>[6x]DRHHHHHHGSVTQRTFKLDYSRDRFLKDGQPFRYISGSIHYFRIPRFYWEDRLLKMKMAGLNAIQMYVPWNFHEPQPGQYEFSGDRDVEHFIQLAHELGLLVILRPGPYICAEWDMGGLPAWLLEKQSIVL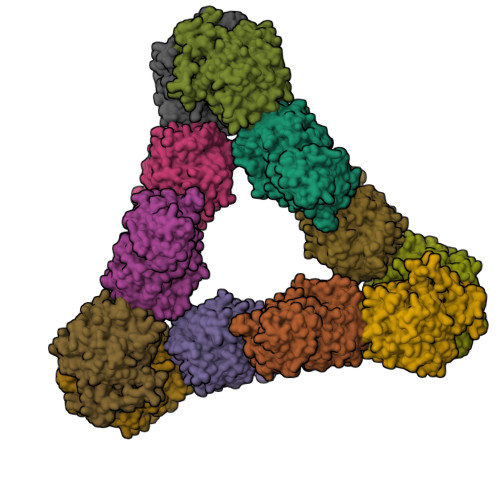RSSDPDYLVAVDKWLAVLLPKMKPLLYQNGGPIITVQVENEYGSYFACDYDYLRFLVHRFRYHLGNDVILFTTDGASEKMLKCGTLQDLYATVDFGTGNNITQAFLVQRKFEPKGPLINSEFYTGWLDHWGKPHSTVKTKTLATSLYNLLARGANVNLYMFIGGTNFAYWNGANTPYEPQPTSYDYDAPLSEAGDLTKKYFALREVIQMFKEVPEGPIPPSTPKFAYGKVALRKFKTVAEALGILCPNGPVKSLYPLTFTQVKQYFGYVLYRTTLPQDCSNPKPIFSSPFNGVRDRAYVSVDGVPQGILDRNLMTALNIQGKAGATLDILVENMGRVNYGRFINDFKGLISNMTINSTVLTNWTVFPLDTEAMVRNHLWGREASDGGHLDGRSTSNSSDLILPTFYVGNFSIPSGIPDLPQDTFIQFPGWSKGQVWINGFNLGRYWPTMGPQKTLFVPRNILTTSAPNNITVLELEFAPCSEGTPELCTVEFVDTPVIS;>[6x]DRHHHHHHGSAPDQDEIDALPGLAKQPSFRQYSGYLRASDSKHFHYWFVESQNDPKNSPVVLWLNGGPGCSSLDGLLTEHGPFLIQPDGVTLEYNPYAWNLIANVLYIESPAGVGFSYSDDKMYVTNDTEVAENNYEALKDFFRLFPEYKDNKLFLTGESYAGIYIPTLAVLVMQDPSMNLQGLAVGNGLASYEQNDNSLVYFAYYHGLLGNRLWTSLQTHCCAQNKCNFYDNKDPECVNNLLEVSRIVGKSGLNIYNLYAPCAGGVPGRHRYEDTLVVQDFGNIFTRLPLKRRFPEALMRSGDKVRLDPPCTNTTAPSNYLNNPYVRKALHIPESLPRWDMCNFLVNLQYRRLYQSMNSQYLKLLSSQKYQILLYNGDVDMACNFMGDEWFVDSLNQKMEVQRRPWLVDYGESGEQVAGFVKECSHITFLTIKGAGHMVPTDKPRAAFTMFSRFLNKEPY> MVHYYRLSLKSRQKAPKIVNSKYNSILNIALKNFRLCKKHKTKKPVQILALLQEIIPKSYFGTTTNLKRFYKVVEKILTQSSFECIHLSVLHKCYDYDAIPWLQNVEPNLRPKLLLKHNLFLLDNIVKPIIAFYYKPIKTLNGHEIKFIRKEEYISFESKVFHKLKKMKYLVEVQDEVKPRGVLNIIPKQDNFRAIV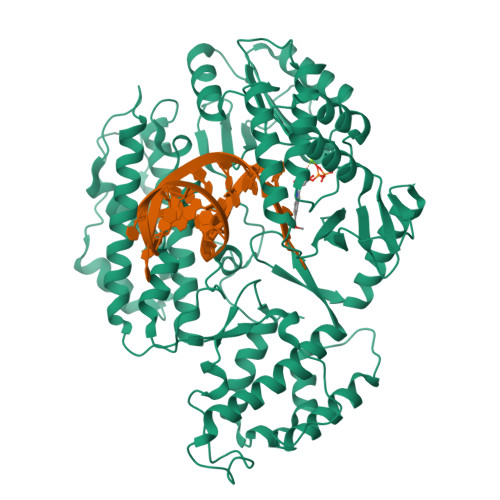SIFPDSARKPFFKLLTSKIYKVLEEKYKTSGSLYTCWSEFTQKTQGQIYGIKVDIRDAYGNVKIPVLCKLIQSIPTHLLDSEKKNFIVDHISNQFVAFRRKIYKWNHGLLQGDPLSGCLCELYMAFMDRLYFSNLDKDAFIHRTVDDYFFCSPHPHKVYDFELLIKGVYQVNPTKTRTNLPTHRHPQDEIPYCGKIFNLTTRQVRTLYKLPPNYEIRHKFKLWNFNNQISDDNPARFLQKAMDFPFICNSFTKFEFNTVFNDQRTVFANFYDAMICVAYKFDAAMMALRTSFLVNDFGFIWLVLSSTVRAYASRAFKKIVTYKGGKYRKVTFQCLKSIAWRAFLAVLKRRTEIYKGLIDRIKSREKLTMKFHDGEVDASYFCKLPEKFRFVKINRKASI>GAMDPREVILCKDQDGKIGLRLKSIDNGIFVQLVQANSPASLVGLRFGDQVLQINGENCAGWSSDKAHKVLKQAFGEKITMTIRDRPFERTITMHKD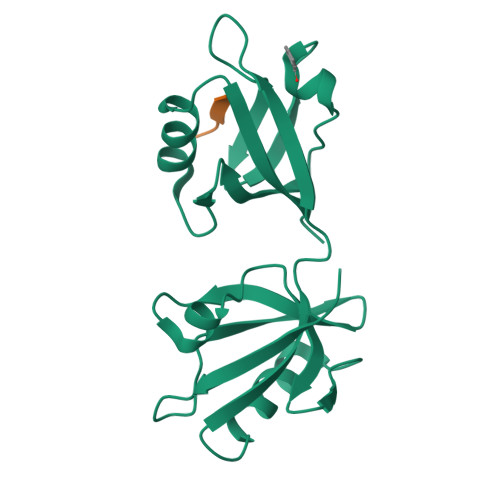STGHVGFIFKNGKITSIVKDSSAARNGLLTEHNICEINGQNVIGLKDSQIADILSTSGTVVTITIMPAF[2x];>[2x]TNEYYV>ATYSTVPKIAFYAGLKRQHEGYEVLKFDDVVTNLGNHYDPTTGKFTCSIPGIYFFTYHVLMRGGDGTSMWADLCKNNQVRASAIAQDADQNYDYASNSVVLHLEPGDEVYIKLDGGKAHGGNNNK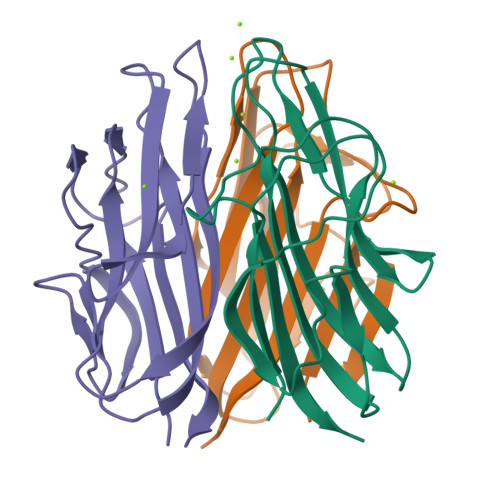YSTFSGFIIYAD[9x]> MRGSHHHHHHGSLVPRGSMVAADAPAAGTDITNQLTNVTVGID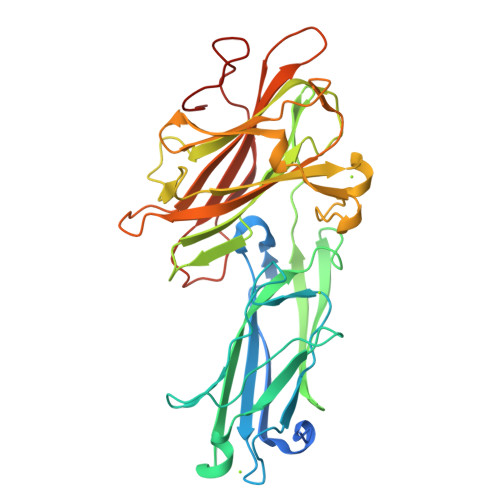SGTTVYPHQAGYVKLNYGFSVPNSAVKGDTFKITVPKELNLNGVTSTAKVPPIMAGDQVLANGVIDSDGNVIYTFTDYVNTKDDVKATLTMPAYIDPENVKKTGNVTLATGIGSTTANKTVLVDYEKYGKFYNLSIKGTIDQIDKTNNTYRQTIYVNPSGDNVIAPVLTGNLKPNTDSNALIDQQNTSIKVYKVDNAADLSESYFVNPENFEDVTNSVNITFPNPNQYKVEFNTPDDQITTPYIVVVNGHIDPNSKGDLALRSTLYGYNSNIIWRSMSWDNEVAFNNGSGSGDGIDKPVVPEQPDEPGEIEPIPEK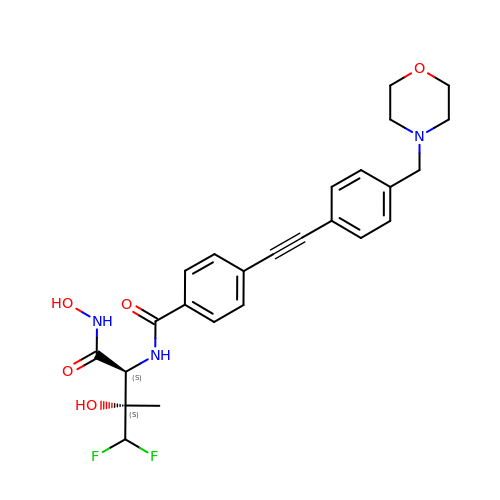N-[(2S,3S)-4,4-difluoro-3-hydroxy-1-(hydroxyamino)-3-methyl-1-oxobutan-2-yl]-4-({4-[(morpholin-4-yl)methyl]phenyl}ethynyl)benzamide | C25 H27 F2 N3 O5 | QNQLYOFTAZBSGC-BWKNWUBXSA-N>[2x]MSGTLLAFDFGTKSIGVAVGQRITGTARPLPAIKAQDGTPDWNIIERLLKEWQPDEIIVGLPLNMDGTEQPLTARARKFANRIHGRFGVEVKLHDERLSTVEARSGLF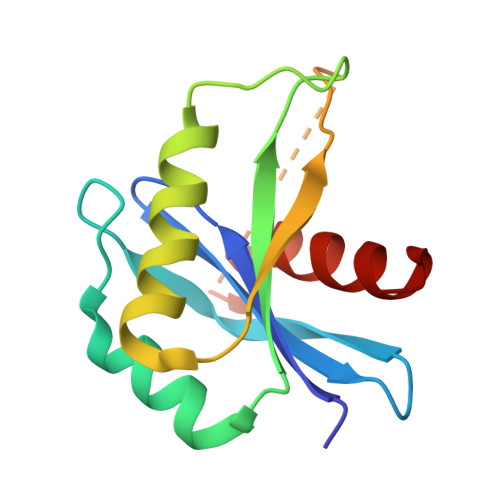EQGGYRALNKGKVDSASAVIILESYFEQGY> MIALSQFNSLSKDEAAGLLAPCVALPAWGETLVSLRPFASRHALLQTAREAMANWGEDELNAALS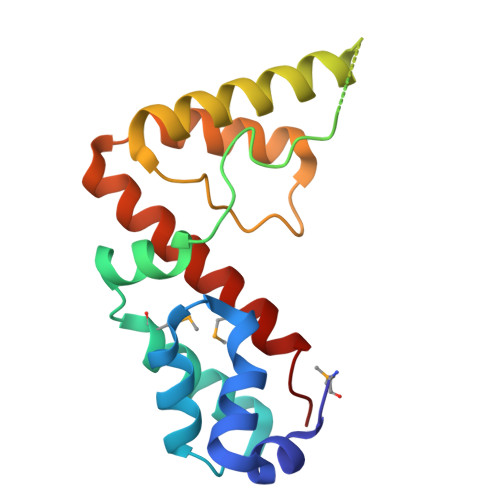AHPRIGEKPTGSQAHAALSRQEQSSVDSENERLAQALREGNARYEARFGRVFLIRAKGRSGEEILQALTRRLQHTADEEVAEALAQLREITMLRLEGAIGE>MKVSLMAAKAKNGVIGCGPHIPWSAKGEQLLFKALTYNQWLLVGRKTFESMGALPNRKYAVVTRSAWTADNDNVIVFPSIEEAMYGLAELTDHVIVSGGGEIYRETLP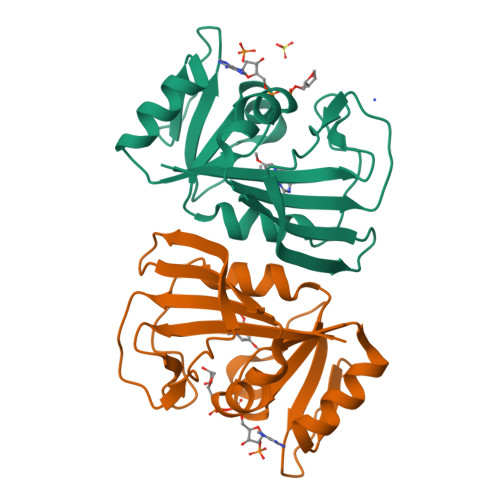MASTLHISTIDIEPEGDVFFPNIPNTFEVVFEQHFSSNINYCYQIWQKG[2x]> GPVEESVDRAVARVADTISSRPTNSESIPALTAAETGHTSQVVPSDTMQTRHVKNYHSRSESSIENFLCRSACVYYATYTNNSKKGFAEWVINTRQVAQLRRKLELFTYLRFDLELTFVITSAQQPSTASSVDAPVQTHQIMYVPPGGPVPTKVKDYAWQTSTNPSVFWTEGNAPPRMSIPFISIGNAYSCFYDGWTQFSRNGVYGINTLNNMGTLYMRHVNEAGQGPIKSTVRIYFKPKHVKAWVPRPPRLCQYEKQKNVNFSPIGVTTSRTDIITT;> SPSAEECGYSDR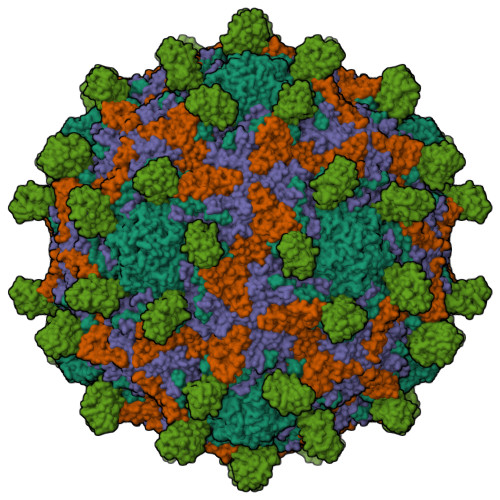VRSITLGNSTITTQECANVVVGYGVWPEYLKDNEATAEDQPTQPDVATCRFYTLESVQWMKNSAGWWWKLPDALSQMGLFGQNMQYHYLGRTGYTIHVQCNASKFHQGCLLVVCVPEAEMGCSNLNNTPEFSELSGGDSARMFTDTQVGESNAKKVQTAVWNAGMGVGVGNLTIFPHQWINLRTNNSATLVMPYINSVPMDNMFRHNNLTLMIIPFVPLNYSEGSSPYVPITVTIAPMCAEYNGLRLASNQ;> GLPVMTTPGSTQFLTSDDFQSPSAMPQFDVTPEMQIPGRVNNLMEIAEVDSVVPVNNTEDNVSSLKAYQIPVQSNSDNGKQVFGFPLQPGANNVLNRTLLGEILNYYTHWSGSIKLTFMFCGSAMATGKFLLAYSPPGAGVPKNRKDAMLGTHVIWDVGLQSSCVLCVPWISQTHYRYVVEDEYTAAGYVTCWYQTNIVVPADVQSSCDILCFVSACNDFSVRMLKDTPFIRQDTFYQ;> MGAQVSTQKTGAHETGLNASGNSVIHYTNINYYKDAASNSANRQDFTQDPGKFTEPVKDIMVKTMPALN;> LSITTPEEMIEKAKGETAYLPCKFTLSPEDQGPLDIEWLISPADNQKVDQVIILYSGDKIYDDYYPDLKGRVHFTSNDLKSGDASINVTNLQLSDIGTYQCKVKKAPGVANKKIHLVVLVK>[5x]SMSNYSVSLVGPAPWGFRLQGGKDFNMPLTISSLKDGGKAAQANVRIGDVV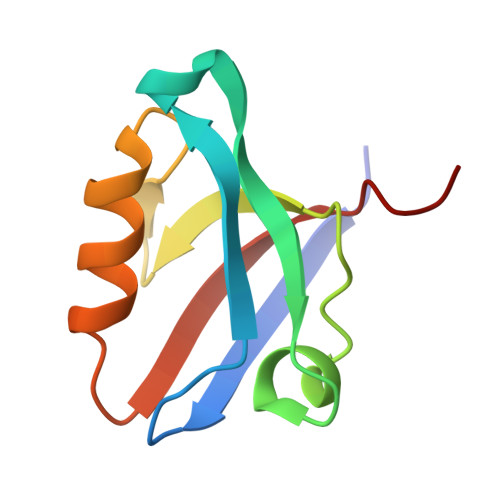LSIDGINAQGMTHLEAQNKIKGCTGSLNMTLQRESDL> AQCSVDIQGNDQMQFNTNAITVDKSCKQFTVNLSHPGNLPKNVMGHNWVLSTAADMQGVVTDGMASGLDKDYLKPDDSRVIAQTKLIGSGEKDSVTFDVSKLK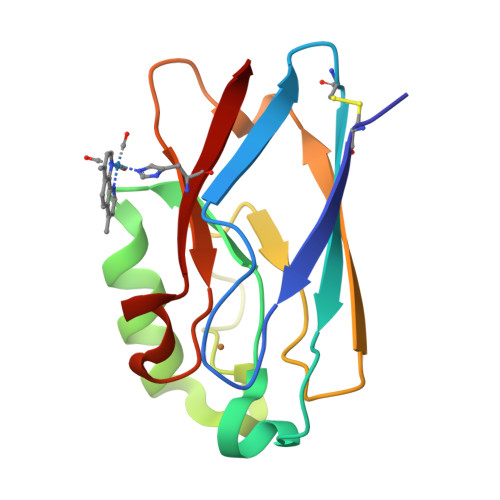EGEQYMFFCTFPGHSALMWGHLTLK>GHMKHTIDPSSPDFQPIPSFEECFPKSTKEHKEVVHEESGHVLKVPFRRVHLSGGEPAFDNYDTSGPQNVNAHIGLAKLRKEWIDRREKLGTPRYTQMYYAKQGIITEEMLYCATREKLDPEFVRSEVARGRAIIPSNKKHLELEPMIVGRKFLVKVNANIGNSAVASSIEEEVYKVQWATMWGADTIMDLSTGRHIHETREWILRNSAVPVGTVPIYQALEKVDGIAENLNWEVFRETLIEQAEQGVDYFTIHAGVLLRYIPLTAKRLTGIVSRGGSIHAKWCLAYHKENFAYEHWDDILDICNQYDVALSIGDGLRPGSIYDANDTAQFAELLTQGELTRRAWEKDVQVMNEGPGHVPMHKIPENMQKQLEWCNEAPFYTLGPLTTDIAPGYDHITSAIGAANIGALGTALLCYVTPKEHLGLPNRDDVKAGVIAYKIAAHAADLAKQHPHAQAWDDALSKARFEFRWMDQFALSLDPMTAMSFHDETLPADGAKVAHFCSMCGPKFCSMKITEDIRKYAEENGYGSAEEAIRQGMDAMSEEFNIAKKTISGEQHGEVGGEIYLPESYVKAAQK[2x]

ThiC, the enzyme discussed here, catalyses the complex rearrangement of aminoimidazole ribonucleotide (AIR) to 4-amino-5-hydroxymethyl-2-methylpyrimidine phosphate (HMP-P) in the thiamin biosynthetic pathways of bacteria and plants 17 and is an example of a non-canonical radical SAM enzyme. The CX2CX4C motif of ThiC varies from the canonical radical SAM motif and is located near the C terminus of the sequence. The homodimeric structure of Caulobacter crescentus ThiC (CcThiC) showed a (β/α)8-barrel fold and suggested that the cluster-binding domain, which was disordered, resides near the C terminus and inserts into the active site of an adjacent protomer through domain swapping. The cluster-binding domain inserts into the active site of an adjacent catalytic domain through domain swapping as previously predicted.

We prepared two different crystal forms of AtThiC, each containing the substrate analogue imidazole ribonucleotide (IRN) and the SAM analogue S-adenosylhomocysteine (SAH), which is also a competitive inhibitor of ThiC21. The mode of SAH binding was unexpected. In the canonical radical SAM enzymes, the SAM amino and carboxylate groups anchor to the differentiated iron in the [4Fe-4S] cluster; however, in ThiC the fourth iron binds to a chloride ion, and the amino and carboxylate groups of SAH anchor to an additional transition metal site. The conformation of SAH is also stabilized by van der Waals interactions and through a salt bridge between the carboxylate and absolutely conserved Arg386. SAH forms two hydrogen bonds with Glu489 through its 2′- and 3′-hydroxyl groups. The adenine base is sandwiched between Leu259 and Met572, the N7 atom forms hydrogen bonds with the guanidinium of Arg343 and the amino group forms a hydrogen bond with the backbone carbonyl of Gly230. In addition to the amino and carboxylate groups of SAH, the metal is coordinated to two absolutely conserved histidine residues (His426 and His490 in AtThiC and His417 and His481 in CcThiC) and two water molecules. Zinc when added to AtThiC at a 1:1 molar ratio during crystallization largely displaces iron at the additional metal site. IRN does not make any direct interactions with SAH.> MRRGPRSLRGRDAPAPTPCVPAECFDLLVRHCVACGLLRTPRPKPAGASSPAPRTALQPQESVGAGAGEAALPLPGLLFGAPALLGLALVLALVLVGLVSWRRRQRRLRGASSAEAPDGDKDAPEPLDKVIILSPGISDATAPAWPPPGEDPGTTPPGHSV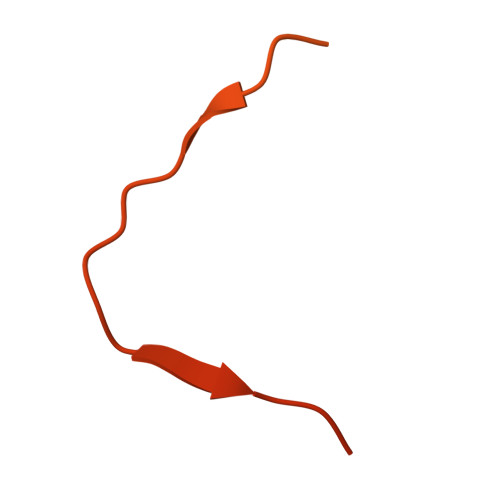PVPATELGSTELVTTKTAGPEQQSNSLEVLFQ>MVRTTKTSMAAASTVAPEVAMDEGSPSTSQAQVELPRNLEVFNEACGHVFGSSFNREDNSVISDAAAFLFKMHTHSLDGQEAKVLRASEKKRERENAKKSRKAPEAGMRVGRSLILTSRWTEYCATCVPALGSKMKVIKASGDAAMIQMMKDHNSLLRVCVRIEVWKARYVSLVALDERIQTLEDAQWFPYLSGDSYRACPGLVGGYFAKKAAAGERGKNYKKLNQTAIIPPPRFLIIGHRLQIGDQVTLRELLASIAWGLCDGVLAECWSPSQGDGSIGVVVGLPLQATGS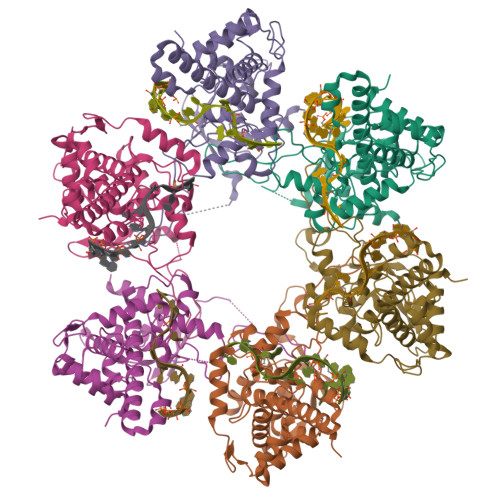CFLVVASHGLSAIADSRIEGTGNTNLLEECIAIQKQDGVIKCKRSGKSLYHCLKETAGAVGR[6x]N-({(2E)-2-[(3-bromophenyl)methylidene]hydrazino}carbonothioyl)-beta-D-glucopyranosylamine | C14 H18 Br N3 O5 S | 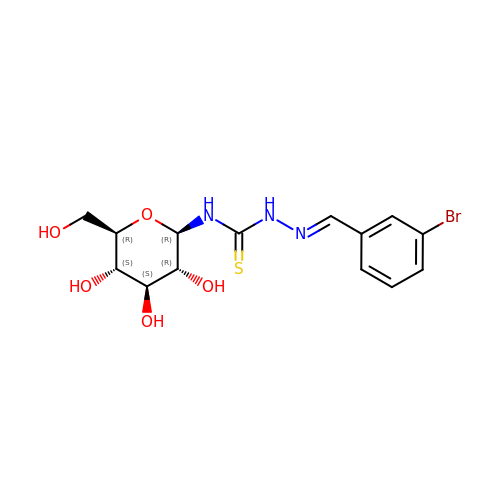PGBHKZPXJWINSR-QCOQDYPWSA-N(4R,4'S)-4,4'-diphenyl-4,4'-biimidazolidine-2,2',5,5'-tetrone 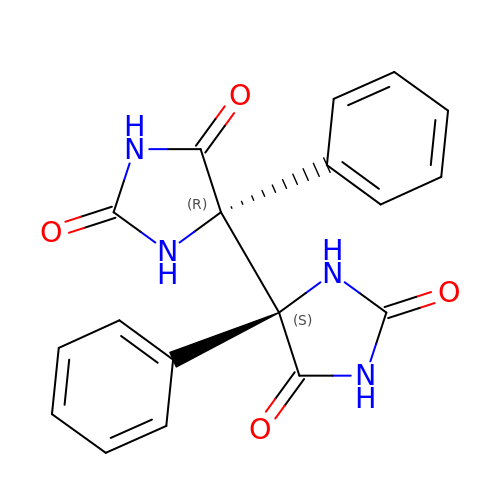| C18 H14 N4 O4 | ZRUGFCSNTLNZEL-HDICACEKSA-N> SALFEPYTLKDVTLRNRIAIPPMCQYMAEDGMINDWHHVHLAGLARGGAGLLVVEATAVAPEGRITPGCAGIWSDAHAQAFVPVVQAIKAAGSVPGIQIAHAGRKASANRPWEGDDHIAADD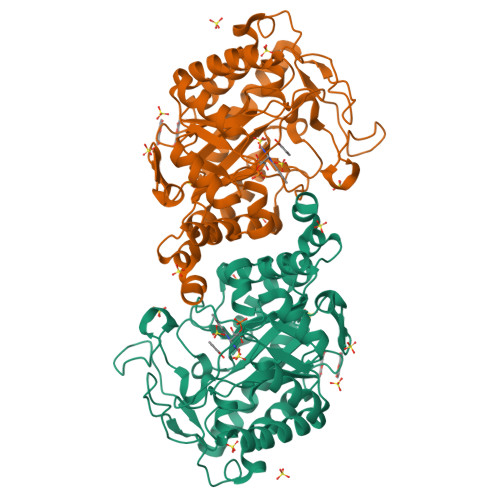TRGWETIAPSAIAFGAHLPKVPREMTLDDIARVKQDFVDAARRARDAGFEWIELHFAHGYLGQSFFSEHSNKRTDAYGGSFDNRSRFLLETLAAVREVWPENLPLTARFGVLEYDGRDEQTLEESIELARRFKAGGLDLLSVSVGFTIPDTNIPWGPAFMGPIAERVRREAKLPVTSAWGFGTPQLAEAALQANQLDLVSVGRAHLADPHWAYFAAKELGVEKASWTLPAPYAHWLE>[4x]MQSDTQ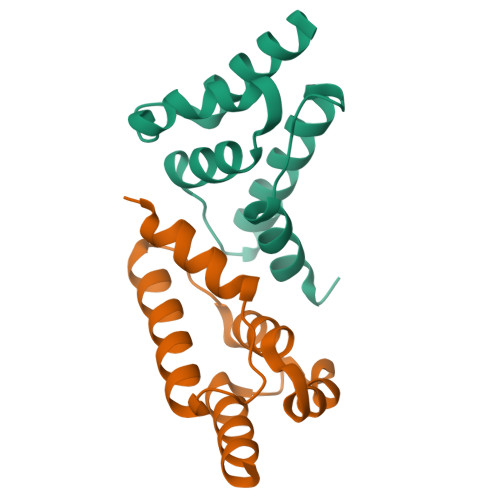EVNDITTLANLHYNGSTPADAFEAEVTNILDRLNNNGIPINNKVACQFIMRGLSGEYRSLRYARSRCINMTVADLFLDIHAIYEEQQEWRRPLEH> EEMKKGHLERECMEETCSYEEAREVFEDSDKTNEFWNKYKDGDQC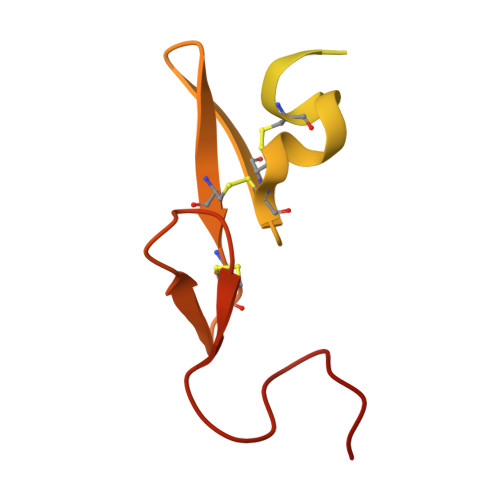ETSPCQNQGKCKDGLGEYTCTCLEGFEGKNCELFTRKLCSLDNGDCDQFCHEEQNSVVCSCARGYTLADNGKACIPTGPYPCGKQTLER>[2x]GSMAAAGRRIPGYRAQVTTEAPAKVVKHSKKQDENIVVNKFKPKEPYVGRCLLNTKITGDDAPGETWHMVFSTEGEVPYREGQSIGIVPDGIDKNGKPHKLRLYSIASSAIGDFGDSKTVSLCVKRVPDGVCSNFLCDLKPGSEVKITGPVGKEMLMPKD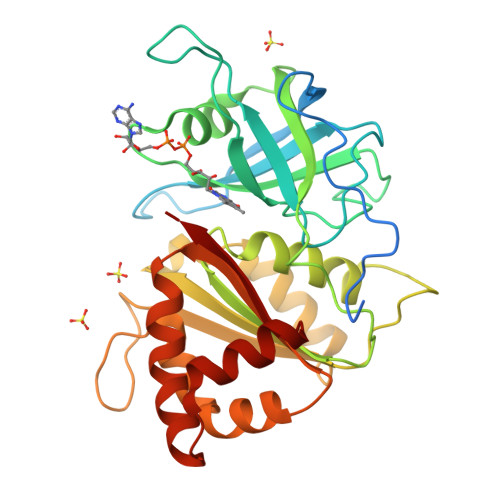PNATVIMLGTGTGIAPFRSFLWKMFFEKHEDYQFNGLAWLFLGVPTSSSLLYKEEFEKMKEKAPENFRLDFAVSREQVNDKGEKMYIQTRMAQYAEELWELLKKDNTFVYMCGLKGMEKGIDDIMVSLAAKDGIDWIEYKRTLKKAEQWNVEVYW1-[(4-phenylphenyl)methyl]-4-pyrrolidin-1-yl-pyridine 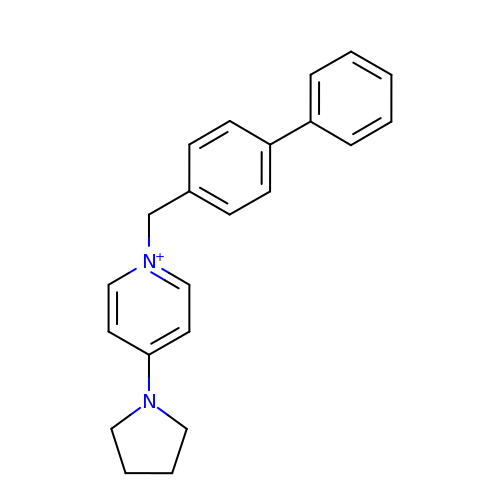| C22 H23 N2 | XOUNRIZMFAXTRS-UHFFFAOYSA-N5-(4,6-dimorpholin-4-yl-1,3,5-triazin-2-yl)-4-(trifluoromethyl)pyridin-2-amine 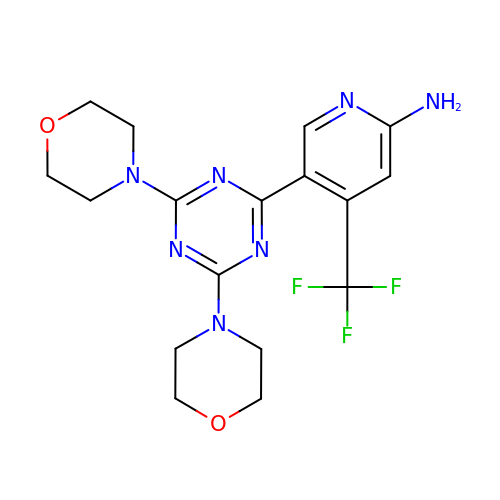| C17 H20 F3 N7 O2 | ADGGYDAFIHSYFI-UHFFFAOYSA-N> GSACGKLTGISDPVTVKTSGSRFGSWMTDPLAPEGDNRVWYMDGYHNNRFVREYKSMV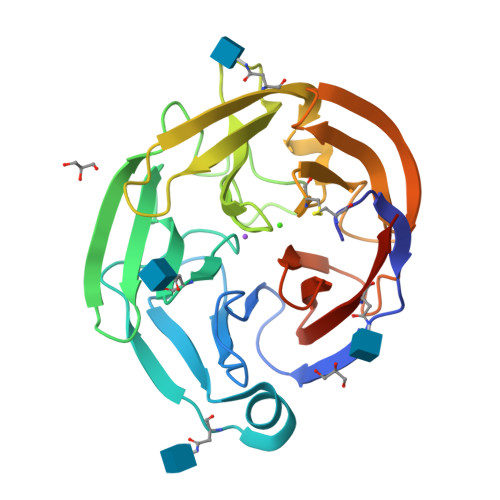DFMNTDNFTSHRLPHPWSGTGQVVYNGSIYFNKFQSHIIIRFDLKTETILKTRSLDYAGYNNMYHYAWGGHSDIDLMVDENGLWAVYATNQNAGNIVISKLDPVSLQILQTWNTSYPKRSAGEAFIICGTLYVTNGYSGGTKVHYAYQTNASTYEYIDIPFQNKYSHISMLDYNPKDRALYAWNNGHQTLYNVTLFHAAAHHHHHH> MAHHGVSGLVGKLVTQLEVNCDADIFYKIVKHHEEVPNVIPHFFTGVQVTKGDGLVSGCIKEWNYVLEGKAMTAVEETTHADETRTLTHHITEGDAMKDYKKFDVIVETNPKPNGHGSVVTYSIVYEKINEDSPAPFDYLKFFHQNIVDMSAHIC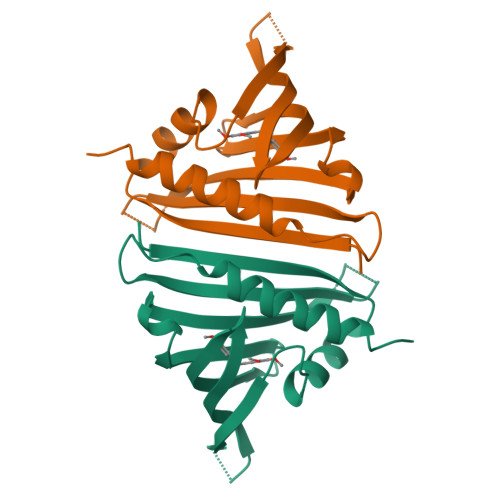SSA>[2x]MTTNLTNS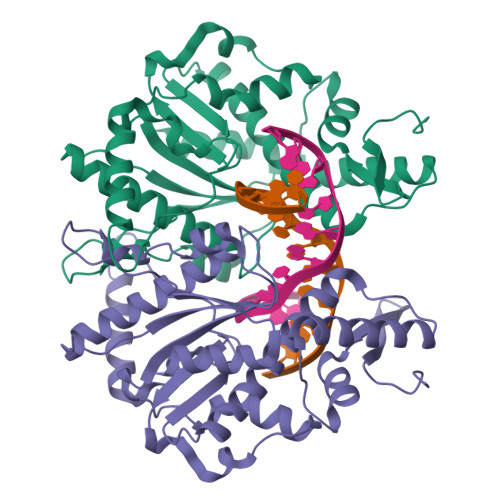NCVEEYKENGKTKIRIKPFNALIELYHHQTPTGSIKENLDKLENYVKDVVKAKGLAIPTSGAFSNTRGTWFEVMIAIQSWNYRVKRELNDYLIIKMPNVKTFDFRKIFDNETREKLHQLEKSLLTHKQQVRLITSNPDLLIIRQKDLIKSEYNLPINKLTHENIDVALTLFKDIEGKCKWDSLVAGVGLKTSLRPDRRLQLVHEGNILKSLFAHLKMAYWNPKAEFKYYGASSEPVSKADDDALQTAATHTIVNVNSTPERAVDDIFSLTSFEDIDKMLDQIIKK>MEFSSPSREECPKPLSRVSIMAGSLTGLLLLQAVSWASGARPCIPKSFGYSSVVCVCNATYCDSFDPPTFPALGTFSRYESTRSGRRMELSMGPIQANHTGTGLLLTLQPEQKFQKVKGFGGAMTDAAALNILALSPPAQNLLLKSYFSEEGIGYNIIRVPMASCDFSIRTYTYADTPDDFQLHNFSLPEEDTKLKIPLIHRALQLAQRPVSLLASPWTSPTWLKTNGAVNGKGSLKGQPGDIYHQTWARYFVKFLDAYAEHKLQ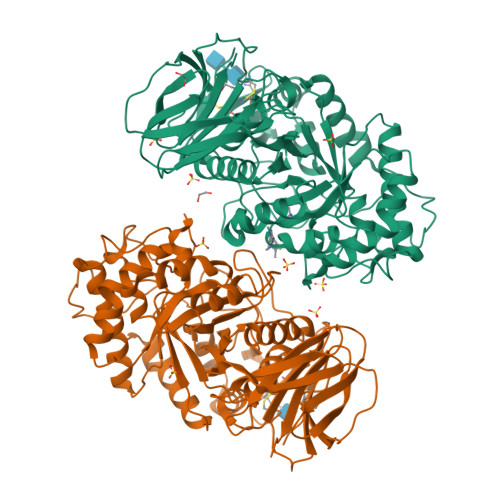FWAVTAENEPSAGLLSGYPFQCLGFTPEHQRDFIARDLGPTLANSTHHNVRLLMLDDQRLLLPHWAKVVLTDPEAAKYVHGIAVHWYLDFLAPAKATLGETHRLFPNTMLFASEACVGSKFWEQSVRLGSWDRGMQYSHSIITNLLYHVVGWTDWNLALNPEGGPNWVRNFVDSPIIVDITKDTFYKQPMFYHLGHFSKFIPEGSQRVGLVASQKNDLDAVALMHPDGSAVVVVLNRSSKDVPLTIKDPAVGFLETISPGYSIHTYLWHRQ[4x]> MMFGRFTERAQKVLALAQEEALRLGHNNIGTEHILLGLVREGEGIAAKALQALGLGSEKIQKEVESLIGRGQEMSQTIHYTPRAKKVIELSMDEARKLGHSYVGTEHILLGLIREGEGVAARVLNNLGVSLNKARQQVLQLLGSNETGSSAAGTNSNANTPTLDSLARDLTAIAKEDSLDPVIGRSKEIQRVIEVLSRRTKNNPVLIGEPGVGKTAIAEGLAQQIINNEVPEILRDKRVMTLDMGTVVAGTKYRGEFEDRLKKVMDEIRQAGNIILFIDALHTLIGAGGAEGAIDASNILKPSLARGELQCIGATTLDEYRKYIEKDAALERRFQPIQVDQPSVDESIQILQGLRDRYEAHHRVSITDDAIEAAVKLSDRYISDRFLPDKAIDLIDEAGSKVRLRSFTTPPNLKELEQKLDEVRKEKDAAVQSQEFEKAASLRDTEQRLREQVEDTKKSWKEKQGQENSEVTVDDIAMVVSSWTGVPVSKIAQTETDKLLNMENILHSRVIGQDEAVVAVAKAVRRARAGLKDPKRPIGSFIFLGPTGVGKTELARALAESIFGDEESMIRIDMSEYMEKHSTSRLVGSPPGYVGYDEGGQLTEKVRRKPYSVVLLDAIEKAHPDVFNILLQVLEDGRLTDSKGRTVDFRNTILIMTSNVGASELKRNKYVGFNVQDETQNHKDMKDKVMGELKRAFRPEFINRIDEIIVFHSLEKKHLTEIVSLMSDQLTKRLKEQDLSIELTDAAKAKV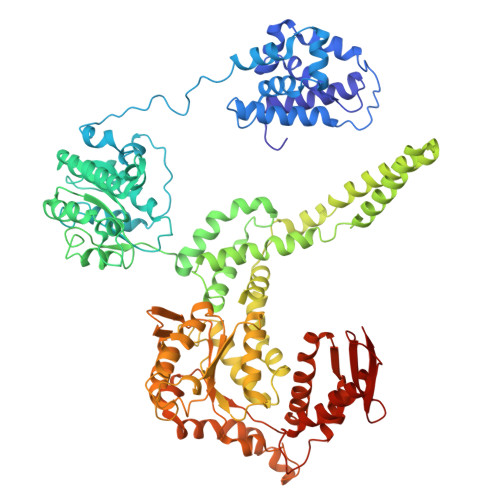AEEGVDLEYGARPLRRAIQKHVEDRLSEELLRGNIHKGQHIVLDVEDGEFVVKTTAKTN> MHLKELLEITDTTERDRSLRRAFSPYTAMIDITGSEAVALIILLNLTYRKNQVDDLLDKKLAKQALKSEDHINKCIKEIAWFHTHNLKYPDIRVSKQNLAVEPPTLHSYVLSSANYPKAYGWSHNSAKVNFAKLFVSYFKWQNQVSWLAQVLATNSDNWKSAFTSLGLSVKAFKSLCVTVKNSLPEEAIPDSVDRYSRQIRMPYHDGYLAVTPVISHVVQSKIQQAAIDKRARFSNVEFTRPAAVSMLAASLGGVINVLNYPPYIRSKYHGLSNSRAFKLNNGQTVFNVEALLKPELIKALEGIIFSNNALALKQRRQQKVKNIKELRNTLLEWFSPVFEWRLDAIENGYDLEQLESASERLEYKILSLPDNELPSLTIPLFRLLNEMLGGVSMTQRYAFHPKLMSPLKAALQWLLVNLTDQKHVLIEEDDEHYRYLHLSGIRVFDAQALSNPYCSGIPSLTAVWGMIHSYQRKLNEALGTNVRFTSFSWFIRNYSAVAGKKLPELSLQGAQQSRLKRPGIIDGKYCDLVFDLIIHIDGYEDDLQAVDSKPDILKAHFPSNFAGGVMHQPELNSNINWCCLYSNENQLFEKLRRLPLSGCWVMPTEHKIQDLDELLLLLNSDSKLSPSMMGYMLLTEPMARVGSLERLHCYAEPAIGVVKYEAATSVRLKGIGNYFNSAFWMLDAQEKFMLMKKV;>MELCNILKYDRSLYPGKAVFFYKTADSDFVPLEADINKIRGPKSGFTEAFTPQFSPKNISPQDLTHNNILTLEECYVPPNVEHIFCRFSLRVQANSLVPSGCSDPEVFSLLKELAETFKECGGYKELAVRYCRNILIGTWLWRNQNTGNTQIEIKTSKGSCYLIDNTRKLAWESKWASDDLKVLEELSNEIESALTDPNVFWSADITAKIEASFCQEIYPSQILNDKVKQGEASKQFVKAKCADGRYAVSFNSVKIGAALQSIDDWWDEDASKRLRVHEFGADKEIGVARRPPDSEQNFYSIFKNTEWYLSALKNCITNKNEKIDPAIYYLFSVLIKGGMFQKKAEAKKA[6x];> MQRYYFTVHFLPKQANLALLTGRCISIMHGFILKHNIEGMGVTFPAWSDSSIGNEIAFVYTDKEILNTLKDQAYFVDMQDCGFFKVSQVLAVPDSC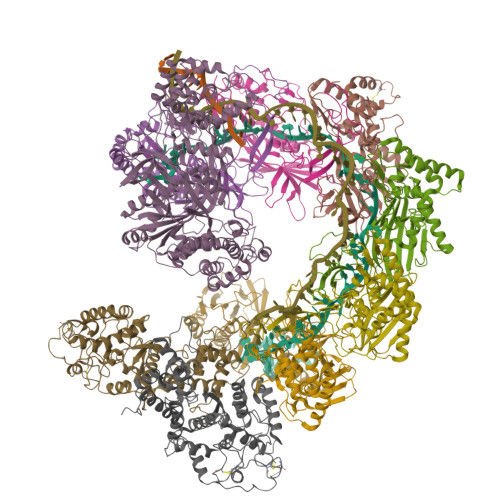EEVRFIRNQAVAKIFTGESRRRLKRLQKRALARGEDFNPKKIEAPREIDIFHRVAMTSKSSQEDYILHIQKQDVDCQAEPYFSNYGLASNEKFKGTVPDLSPSIDRN;>MGHHHHHHHHHHGGSENLYFQSGMAFLFSPKARAFSDESLESYLLRVVSENFFDSYEGLSLAIREELHELDFEAHGAFPVDLKRLNVYHAKHNSHFRMRALGLLETLLDLPRYELQKLALLKSDIKFNSSVALYNNGVDIPLRFIRHHAEEAVDSIPVCSQCLAEEAYIKQSWHIKWVNACTKHQCALLHNCPECYAPINYIENESITHCSCGFELSCASTSPVNTLSIEHLNKLLDKGERNDSNPLFNNMTLTERFAALLWYQERYSQTDNFCLNDAVNYFSKWPAVFNTELDELSKNAEMKLIDLFNKTEFKFIFGDAILACPSTQKQSESHFIYRALLDYLVTLVESNPKTKKPNAADLLVSVLEAATLLGTSVEQVYRLYQNGILQTAFRHKMNQRINPYKGAFFLRHVIEYKTSFGNDKARMYLSAW[2x]> MAGAPHPHTYMGWWGSLGSPKQKYITQYTISPYAAKPLKGAAYNAVFNTFRRTKNQFLY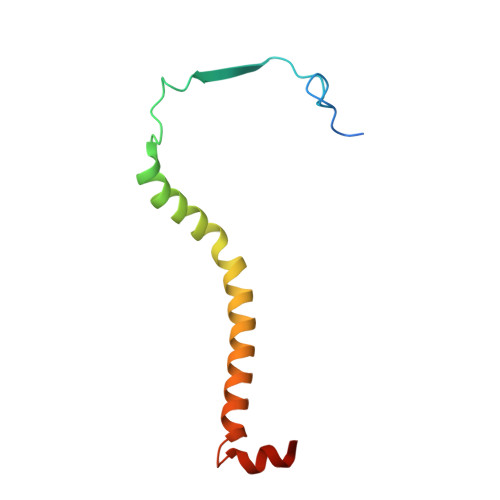VAIPFVVVWSIWTRARDYNEYLYTKEGREELERVNV> SMAVEPKEDTITVTAAPAPQESAWGPAATIAARQSATGTKTDTPIQKVPQSISVVTAEEMALHQPKSVKEALSYTPGVSVGTRGASNTYDHLIIRGFAAEGQSQNNYLNGLKLQGNFYNDAVIDPYMLERAEIMRGPVSVLYGKSSPGGLLNMVSKRPTTEPLKEVQFKAGTDSLFQTGFDFSDSLDDDGVYSYRLTGLARSANAQQKGSEEQRYAIAPAFTWRPDDKTNFTFLSYFQNEPETGYYGWLPKEGTVEPLPNGKRLPTDFNEGAKNNTYSRNEKMVGYSFDHEFNDTFTVRQNLRFAENKTSQNSVYGYGVCSDPANAYSKQCAALAPADKGHYLARKYVVDDEKLQNFSVDTQLQSKFATGDIDHTLLTGVDFMRMRNDINAWFGYDDSVPLLNLYNPVNTDFDFNAKDPANSGPYRILNKQKQTGVYVQDQAQWDKVLVTLGGRYDWADQESLNRVAGTTD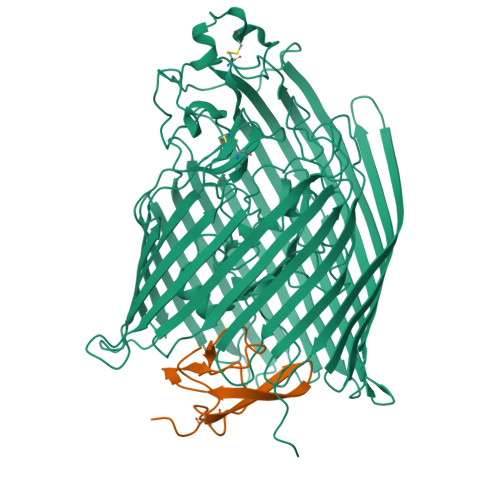KRDDKQFTWRGGVNYLFDNGVTPYFSYSESFEPSSQVGKDGNIFAPSKGKQYEVGVKYVPEDRPIVVTGAVYNLTKTNNLMADPEGSFFSVEGGEIRARGVEIEAKAALSASVNVVGSYTYTDAEYTTDTTYKGNTPAQVPKHMASLWADYTFFDGPLSGLTLGTGGRYTGSSYGDPANSFKVGSYTVVDALVRYDLARVGMAGSNVALHVNNLFDREYVASCFNTYGCFWGAERQVVATATFRF;> MKKLFLAMAVVLLSACSTFGPKDIKCEAYYMQDHVKYKANVFDRKGDMFLVSPIMAYGSFWAPVSYFTEGNTCEGVFHHHHHH> FRASCTLLGHGQYKTRLKKRMVGFIPKVIPRKIRNNMVALRSEANTGHMEGYIKTEAERLDATGRKLQKTMWDPVLQRYTLMKETKVRGPFLTKSN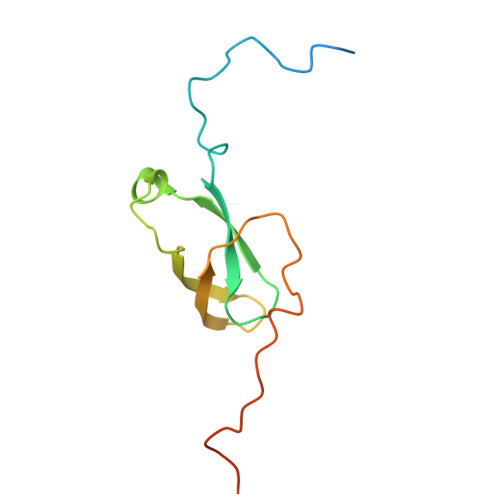IARKVDFPVGALHGTKLGGKK>MTDQVFGKVSKVVCVGAGYVGGPTCAMIAHKCPHITVTVVDMNTAKIAEWNSDKLPIYEPGLDEIVFAARGRNLFFSSDIPKAIAEADLIFISVNTPTKMYGRGKGMAPDLKYVESVSRTIAQYAGGPKIVVEKSTVPVKAAESIGCILREAQKNNENLKFQVLSNPEFLAEGTAMKDLANPDRVLIGGESSPEGLQAVAELVRIYENWVPRNRIITTNTWSSELSKLVANAFLAQRISSINSISAVCEATGAEISEVA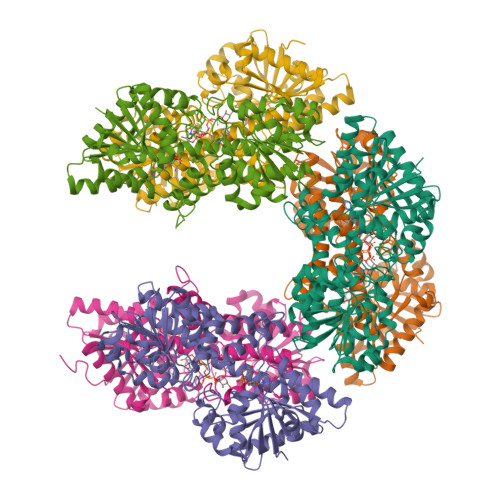HAVGYDTRIGSKFLQASVGFGGSCFQKDVLSLVYLCESLNLPQVADYWQGVININNWQRRRFADKIIAELFNTVTDKKIAIFGFAFKKNTGDTRESSAIHVIKHLMEEHAKLSVYDPKVQKSQMLNDLASVTSAQDVERLITVESDPYAAARGAHAIVVLTEWDEFVELNYSQIHNDMQHPAAIFDGRLILDQKALREIGFRTFAIGTSPDQAYNLFGTAGY[12x]> GSGSNPNVDMTGWEVKLPADLIKDSSGKSQQEVNNSLKLKTFDDLRNFKPIVNGQTVYVGQRSNTYLQGGGLFYADTSDTTSLDNDGTILVGIDGTRWKRKWNTHADPCWFGADYTGTEDCSAQVQKAVDVSYGRVWFGNADRSFKMMTPVGLPTNSIVGDMLMEICGDGARVWVYSNTGIFTSKRSIGLETSTDDLYTAALEIGRGLRFQGDGVSQSVVVNGDRLYNVNMKGGRYLRISALVRATQPRRNETTGYVQSVTIEENHLALCNRIIDSKRGFNVTVS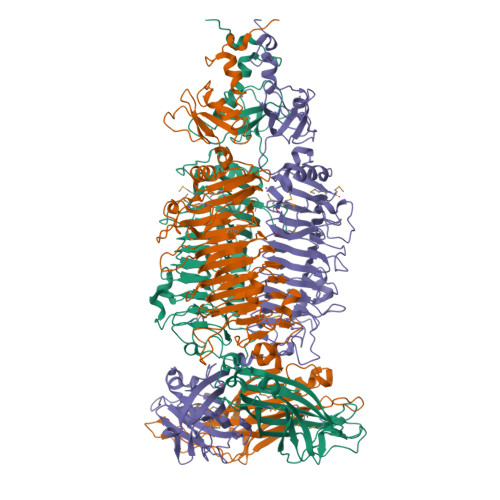RNFCESCYGGVYLDGDGSPAVNVIRCDGNLWESSGVFAKLGAVYAGTFIGNYFEGNNTGDLPTLKCLIELGKTGTTGYSSGVTFIGNQFGAAAAYKADVNYADVKFTASLSGTNLDVLAPPTFVGNWTNAYRMWSEGQVVTQFGNAFSGGNARRHQAPKLHTEARVTFDLSRKEFLSSTNLVGGVHTVAEIDTNLISNLASQSSRACTADMNIFMQMKTASNVVLGAAVAKVSLVVQGSEGIGTGATTDVYVAASLTGFTQLEGGVIDTVNNVSLFKHFTSPVLTIERVGTKYLLKLSGYVAASGSLYGATAKVFSSTTMTIYSLNSGASVAGQIYPT>MVAVEQSEASRLGPVFDSCRANNRAALIGYLPTGYPDVPASVAAMTALVESGCDIIEVGVPYSDPGMDGPTIARATEAALRGGVRVRDTLAAVEAISIAGGRAVVMTYWNPVLRYGVDAFARDLAAAGGLGLITPDLIPDEAQQWLAASEEHRLDRIFLVAPSSTPERLAATVEASRGFVYAASTMGVTGARDAVSQAAPELVGRVKAVSDIPVGVGLGVRSRAQAAQIAQYADGVIVGSALVTALTEGLPRLRALTGELAAGVRLGMSAHHHHHH[4x];>MSAAIAEPTSHDPDSGGHFGGPSGWGGRYVPEALMAVIEEVTAAYQKERVSQDFLDDLDRLQANYAGRPSPLYEATRLSQHAGSARIFLKREDLNHTGSHKINNVLGQALLARRMGKTRVIAETGAGQHGVATATACALLGLDCVIYMGGIDTARQALNVARMRLLGAEVVAVQTGSKTLKDAINEAFRDWVANADNTYYCFGTAAGPHPFPTMVRDFQRIIGMEARVQIQGQAGRLPDAVVACVGGGSNAIGIFHAFLD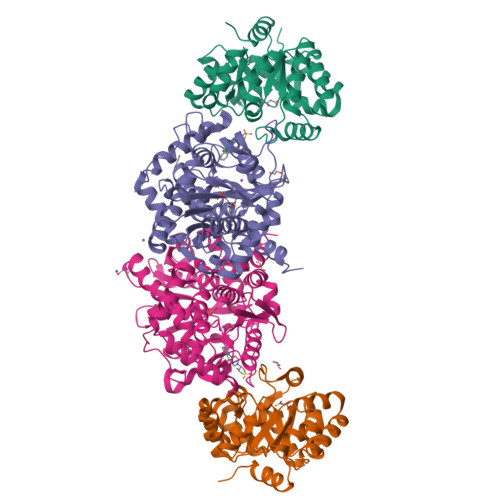DPGVRLVGFEAAGDGVETGRHAATFTAGSPGAFHGSFSYLLQDEDGQTIESHSISAGLDYPGVGPEHAWLKEAGRVDYRPITDSEAMDAFGLLCRMEGIIPAIESAHAVAGALKLGVELGRGAVIVVNLSGRGDKDVETAAKWFGLLGND[4x]> MNASTAAVNSIGMVPTVGTPVNINVNASNPLLHPHLDDPSLLNNPIWKLQLHLAAVSAQSLGQPNIYARQNAMKKYLATQQAQQAQQQAQQQAQQQVPGPFGPGPQAAPPALQPTDFQQSHIAEASKSLVDCTKQALMEMADTLTDSKTAKKQQPTGDSTPSGTATNSAVSTPLTPKIELFANGKDEANQALLQHKKLSQYSIDEDDDIENRMVMPKDSKYDDQLWHALDLSNLQIFNISANIFKY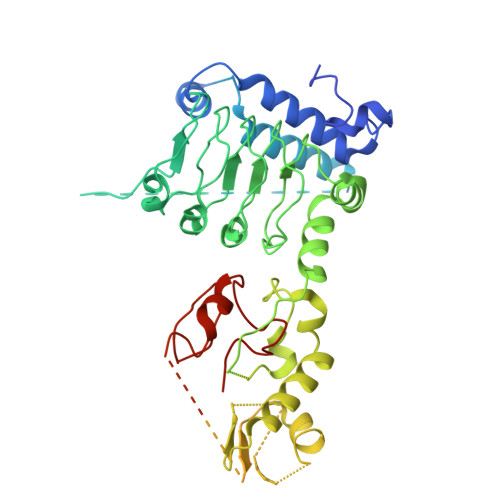DFLTRLYLNGNSLTELPAEIKNLSNLRVLDLSHNRLTSLPAELGSCFQLKYFYFFDNMVTTLPWEFGNLCNLQFLGVEGNPLEKQFLKILTEKSVTGLIFYLRDNRPEIPLPHERRFIEINTDGEPQREYDSLQQSTEHLATDLAKRTFTVLSYNTLCQHYATPKMYRYTPSWALSWDYRRNKLKEQILSYDSDLLCLQEVESKTFEEYWVPLLDKHGYTGIFHAKARAKTMHSKDSKKVDGCCIFFKRDQFKLITKDAMDFSGAWMKHKKFQRTEDYLNRAMNKDNVALFLKLQHIPSGDTIWAVTTHLHWDPKFNDVKTFQVGVLLDHLETLLKEETSHNFRQDIKKFPVLICGDFNSYINSAVYELINTGRVQIHQEGNGRDFGYMSEKNFSHNLALKSSYNCIGELPFTNFTPSFTDVIDYIWFSTHALRVRGLLGEVDPEYVSKFIGFPNDKFPSDHIPLLARFEFMKTNTGSKKV> GSHMN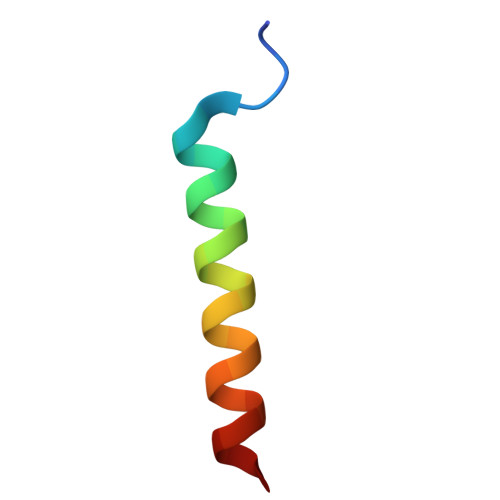LLNAATALSGSMQYLLNYVNAG> MAPSQASHTPSLATWTKSLRDQSLEASIESLIFLLKRRQVTGDECAGAIAQLLRQVVAKSKWHDVDQLLYRVQTAGARLARAAPHEPVIGNIVRRVLGLIRDEASENRNADDIASDAASDIQSLAPSQPPPQQRPPPPARTLTSGLQVSKSMFNLLSVADPSESPVTGASTPISQAQQPFSVHALRSEVMDGIEEILDEINQADDQIASFAEIQIHPGDYVLAYQPSKTVERFLVKAASKRRFTVILASLNPPAPGEEEQPYAALRKKLNAAGVSTINLASNGLMAYIPRVNKVIFGAKAVYQNGGLLVDSGACIAAQAAHEYLKPVIALCGVYKFCPEDPSDEVSRGE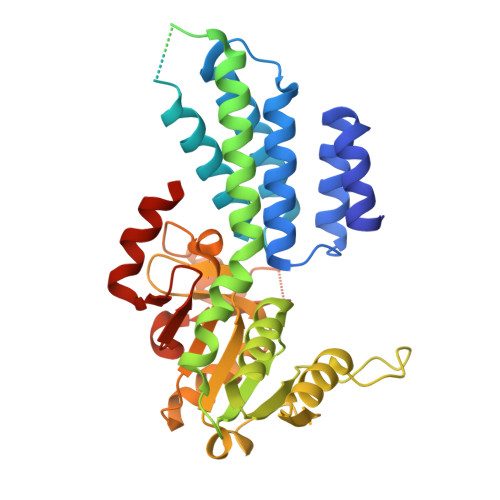LGNPSSYVSYADGPELDSFEVENTTTDYIPPDLVDVYLTNLGPQTRHHLGGIYADHYKIEDIGFSLQVGE>[7x]VEYKNTICPPRQDYRYWYFVAELTIGVNYDINSTIIGECHMSESYIDRNANIVLTGYGLKINMTIMDTDQRFVAAAEGVGKDNKLSVLLFTTQRLDKVHHNISVTITCMEMNCGTTKYNSDLPESIHKSSSCDITINGSCVTCVNLETDPTKINPHYLHPKNKYLYHNSEYSMRGSYGVTFIDELNQCLLDIKELSYDICYRE;>LKIQAYFNETADLPCQFANSQNQSLSELVVFWQDQENLVLNEVYLGKEKFDSVHSKYMGRTSFDSDSWTLRLHNLQIKDKGLYQCIIHHKKPTGMIRIHQMNSELSVLANFSQPEIVPISNITENVYINLTCSSIHGYPEPKKMSVLLRTKNSTIEYDGVMQKSQDNVTELYDVSISLSVSFPDVTSNMTIFCILETDKTRLLSSPFSIELED[7x]

Poxvirus encoded M2 protein is a member of the poxvirus immune evasion family and plays roles in host immunomodulation via the regulation of innate immune response mediated by the NF-κB pathway and adaptive immune response mediated by B7 ligands. Here we reveal that MPXV M2, co-existing as a hexamer and a heptamer, recognizes human B7.1 and B7.2 (hB7.1/2) with high avidities. The binding of oligomeric MPXV M2 interrupts the interactions of hB7.1/2 with CD28 and CTLA4 and subverts T cell activation mediated by B7.1/2 costimulatory signals. Cryo-EM structures of M2 in complex with hB7.1/2 show that M2 binds to the shallow concave face of hB7.1/2 and displays sterically competition with CD28 and CTLA4 for the binding to hB7.1/2.

Interestingly, two oligomeric states, hexamer and heptamer, were revealed in both cryo-EM samples, which were also observed in 2D class averages of M2 alone. We finally determined three complex structures, M2-hB7.1 hexamer, M2-hB7.2 hexamer, and M2-hB7.2 heptamer, at an overall resolution of 3.04, 2.7, and 3.12 Å, respectively. Unexpectedly, the cryo-EM analysis shows that M2 displays as hexamers and heptamers and binds to hB7.1/2 with both 6:6 and 7:7 stoichiometries. The resulting structures reveal that M2 forms an oligomeric ring structure with B7 proteins binding to the outer face of the M2 ring in a 1:1 stoichiometry. Despite the different oligomeric conformations, the overall structure of each M2 subunit and inter-subunit interactions from hexamer and heptamer structures are virtually identical. The root-mean-square deviation (r.m.s.d) is ~0.4 Å for all Cα atoms of M2 subunits of two oligomeric structures. The subtle differences arise from connecting loops that appear more dynamic owing to fewer protein-protein interactions. We found that the oligomeric M2 proteins can engage into hB7.1/2 with higher avidities than the monovalent interactions of M2 with hB7.1/2.>AECSVDIQGNDQMQFNTNAITVDKSCKQFTVN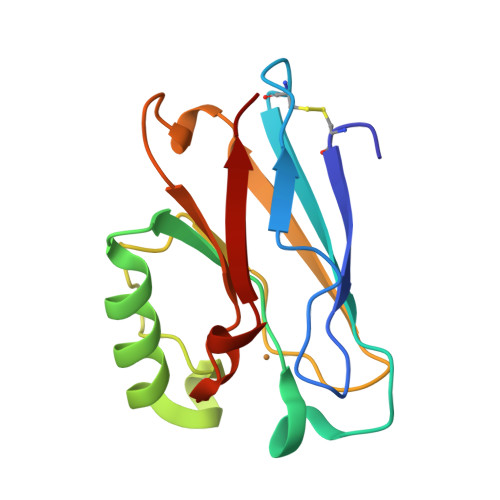LSHPGNLPKNVMGHNWVLSTAADMQGVVTDGMASGLDKDYLKPDDSRVIAHTKLIGSGEKDSVTFDVSKLKEGEQYMFFCTPPGHSALQKGTLTLK[4x]>MIVFVRFNSSHGFPVEVDSDTSIFQLKEVVAKRQGVPADQLRVIFAGKELRNDWTVQNCDLDQQNIVHIVQRPWRKGQEMNATNSFYVYCKGPCQRVQPGKLRVQCSTCRQATLTLTQGPSCWDDVLIPNRMSGECQSPHCPGTSAEFFFKCGAHPTSDKETSVALHLIATNSRNITCITCTDVRSPVLVFQCNSRHVICLDCFHLYCVTRLNDRQFVHDPQLGYSL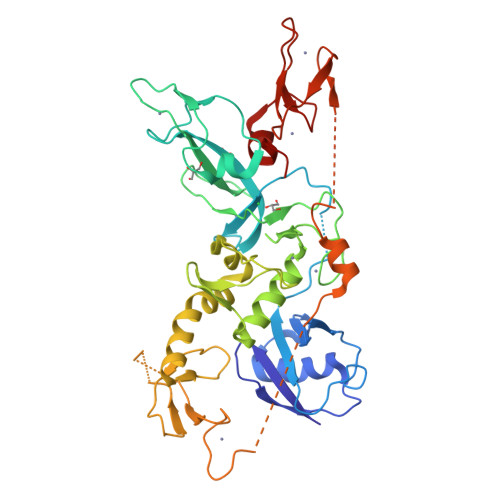PCVAGCPNSLIKELHHFRILGEEQYNRYQQYGAEECVLQMGGVLCPRPGCGAGLLPEPDQRKVTCEGGNGLGCGFAFCRECKEAYHEGECSAVFEASGTTTQAYRVDERAAEQARWEAASKETIKKTTKPCPRCHVPVEKNGGCMHMKCPQPQCRLEWCWNCGCEWNRVCMGDHWFDV[2x]> MIKSTDRKLVVGLEIGTAKVSALVGEILPDGMVNIIGVGNCPSRGMDKGGVNDLESVVKCVQRAIDQAELMADCQISSVYLALSGKHISCQNEIGMVPVSEEEVTQDDVDSVVHTAKSVRVRDEHRILHVIPQEYAIDYQEGIKNPVGLSGVRMQAKVHLITCHNDMAKNIVKAVERCGLKVDQLIFAGLAASYAVLTEDERELGVCVVDIGGGTMDVAVYTGGALRHTKVIPYAGNVVTSDIAYAFGTPPSDAETIKV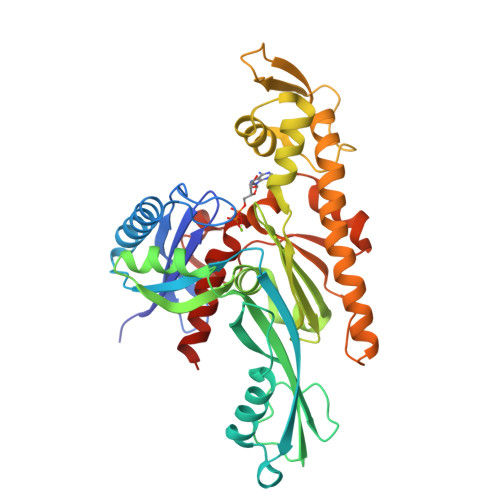RHGCALGSIVSKDESVEVPSVGGRPPRSLQRQTLAEVIEPRYTELLNLVNDEILRLQEQLRQQGVKHHLAAGIVLTGGGAQIDGLAECAQRVFHTQVRIGRPLNITGLTDYVQAPCYSTAVGLLHYGKESHLGGDSD>GSKEGEYIKLKVIGQDSSEIHFKVKMTTHLKKLKESYAQRQGVPMNSLRFLFEGQRIADNHTPKELGMEEEDVIEVYQEQTGG[2x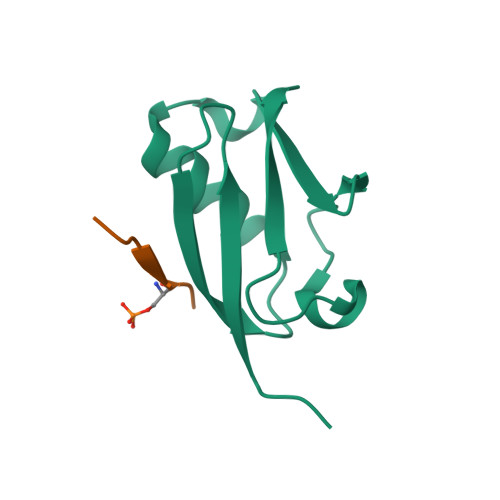];>[2x]GSGEAEERIISLD> EA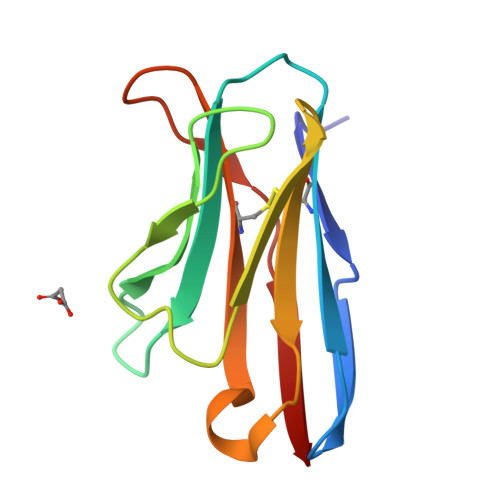AVTQSPRNKVAVTGEKVTLSCQQTNNHNNMYWYRQDTGHGLRLIHYSYGAGNTEKGDIPDGYKASRPSQEQFSLILESATPSQTSVYFCASGGGGTLYFGAGTRLSVL> LTAKHRPSVVWLHNAECVGCTEAAIRTIKPYIDALILDTISLDYQETIMAAAGEAAEAALHQALEGKDGYYLVVEGGLPTIDGGQWGMVAGHPMIETTKKAAAKAKGIICIGTCSAYGGVQKAKPNPSQAKGVSEALGVKTINIPG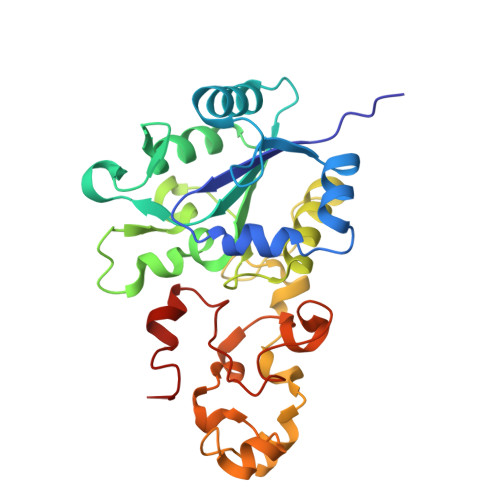CPPNPINFVGAVVHVLTKGIPDLDENGRPKLFYGELVHDNCPRLPHFEASEFAPSFDSEEAKKGFCLYELGCKGPVTYNNCPKVLFNQVNWPVQAGHPCLGCSEPDFWDTMTPFYEQG>[2x]GAMGSARRINDEIERQLRRDKRDARRELKLLLLGTGESGKSTFIKQMRIIHGSGYSDEDKRGFTKLVYQNIFTAMQAMIRAMDTLKIPYKYEHNKAHAQLVREVDVEKVSA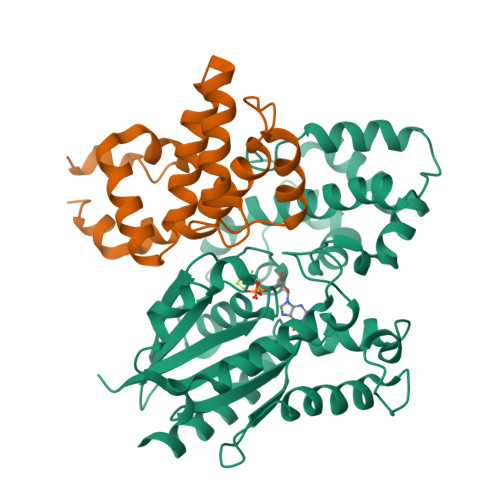FDVPDYAAIKSLWNDPGIQECYDRRREYQLSDSTKYYLNDLDRVADPSYLPTQQDVLRVCVPTTGIIEYPFDLQSVIFRMVDVGGQRSERRKWIHCFENVTSIMFLVALSEYDQVLVESDNENRMEESKALFRTIITYPWFQNSSVILFLNKKDLLEEKIMYSHLVDYFPEYDGPQRDAQAAREFILKMFVDLNPDSDKIIYSHFTCATDTENIRFVFAAVKDTILQLNLKEYNLV;>[2x]GEFGSPSPEEAQLWSEAFDELLASKYGLAAFRAFLKSEFCEENIEFWLACEDFKKTKSPQKLSSKARKIYTDFIEKEAPKEINIDFQTKTLIAQNIQEATSGCFTTAQKRVYSLMENNSYPRFLESEFYQDLCKKPQ> MTAVADAPQADIEGVASPQAVVVGVMAGEGVQIGVLLDANAPVSVMTDPLLKVVNSRLRELGEAPLEATGRGRWALCLVDGAPLRATQSLTEQDV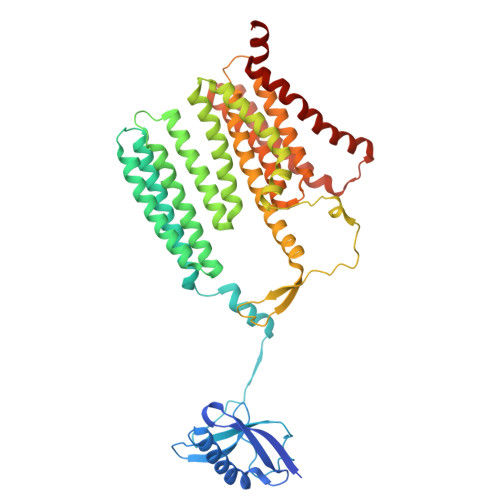YDGDRLWIRFIADTERRSQVIEHISTAVASDLSKRFARIDPIVAVQVGASMVATGVVLATGVLGWWRWHHNTWLTTIYTAVIGVLVLAVAMLLLMRAKTDADRRVADIMLMSAIMPVTVAAAAAPPGPVGSPQAVLGFGVLTVAAALALRFTGRRLGIYTTIVIIGALTMLAALARMVAATSAVTLLSSLLLICVVAYHAAPALSRRLAGIRLPVFPSATSRWVFEARPDLPTTVVVSGGSAPVLEGPSSVRDVLLQAERARSFLSGLLTGLGVMVVVCMTSLCDPHTGQRWLPLILAGFTSGFLLLRGRSYVDRWQSITLAGTAVIIAAAVCVRYALELSSPLAVSIVAAILVLLPAAGMAAAAHVPHTIYSPLFRKFVEWIEYLCLMPIFPLALWLMNVYAAIRYR>MAVKEATSETKKRSGYEIITLTSWLLQQEQKGIIDAELTIVLSSISMACKQIASLVQRANISNLTGTQGAVNIQGEDQKKLDVISNEVFSNCLRSSGRTGIIASEEEDVPVAVEESYSGNYIVVFDPLDGSSNLDAAVSTGSIFGIYSPNDECLPDFGDDSDDNTLGTEEQRCIVNVCQPGSNLLAAGYCMYSSSVIFVLTIGKGVFVFTLDPLYGEFVLTQENLQIPKSGKIYSFNEGNYKLWDENLKKYIDDLKEPGPSGKPYSARYIGSLVGDFHRTLLYGGIYGYP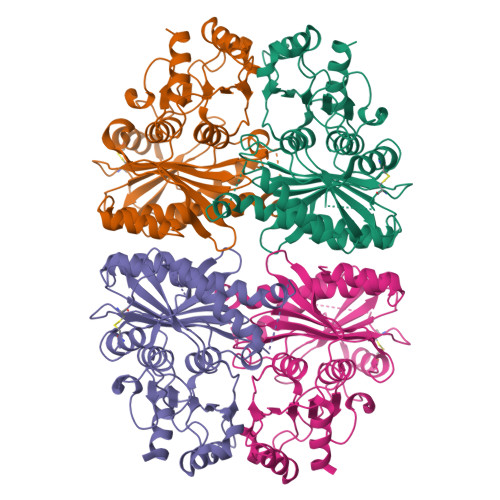RDKKSKNGKLRLLYECAPMSFIVEQAGGKGSDGHQRVLDIQPTEIHQRVPLYIGSTEEVEKVEKYLA[4x]>[4x]MDVPT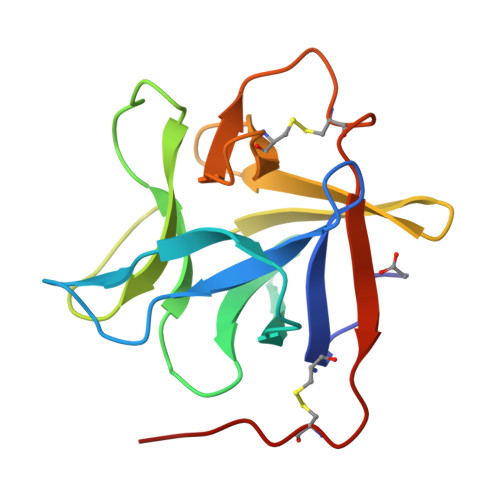GCVTLKFVNNAKHINMWDKTVLHYRKLYGGDEKEEWVIEKSGNDYKIRPRIYTEYLYAESKTDDPGRAVKTLKEGTTDANVWKVEQKMALYWISNVKYQECLVISGSDHVVTKKMDSCGDDLWEIQPVSNCLIVGKKN>[2x]MGSDKIHHHHHHENLYFQGMWKSISQVLAEQFGAYYFIKHKEKLY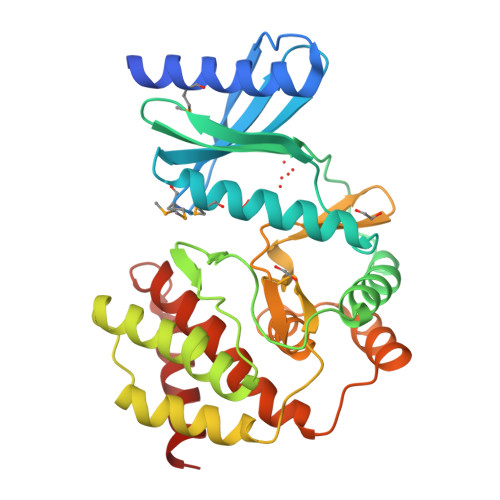SGEMNEIWLINDEVQTVFVKINERSYRSMFRAEADQLALLAKTNSINVPLVYGIGNSQGHSFLLLEALNKSKNKQSSFTIFAEKIAQLHQIQGPDKYGLDFDTWLGPIYQPNDWQTSWAKFFSENRIGWQLQICKEKGLIFGNIDLIVQIVADTLSKHNPKPSILHGNLWIENCIQVDDKIFVCNPACYWGDRECDIAFSSLFEPFPTNFYQRYNEIYPLEEGYLERKLIYQLYYLLNFSYRYYNKKQSYVSLTQKLINQILHKIDK BC-producing bacteria have a cellulose synthase operon in their genome. BcsC consists of about 20–30 residues of signal peptides, followed by about 750–900 residues of periplasmic domain of tetratrico peptide repeat (BcsC-TPR), and about 380 residues of the outer membrane domain of the β-barrel (BcsC-C). Thus, the TPR domain is believed to be important for exporting polysaccharides.

In this report, we determined the crystal structure of the N-terminal six TPR motifs in BcsC (BcsC-TPR(N6), Asp24–Arg272) from Enterobacter CJF-002. The crystal structure of BcsC-TPR (Asp24–Arg272) was determined at a resolution of 3.27 Å. There were five molecules in the asymmetric unit and the Matthew’s coefficient was calculated to be 3.9 Å3 Da−1 with a solvent content of 68.5%26. BcsC-TPR(Asp24–Arg272) is a helical structure formed by 14 α-helices (α1–α14). We found a non-TPR α-helix was inserted in the middle of TPR motifs in this structure. A comparison of five monomers in the asymmetric unit showed that they can be classified into three different conformations: chains A and C were type 1 (root mean square deviation (r.m.s.d.) was 0.74 Å for 243 Cα atoms), chains B and D were type 2 (r.m.s.d. was 0.38 Å for 204 Cα atoms), and chain E was type 3. The conformations of these three types were different at the turn region between α5 and α6. The C-terminal two helices (α12–α13) were not included for this calculation since this region was not built for chain E. These results indicate that BcsC-TPR(N6) consists of two structural domains, an N-terminal TPR domain (α1–α5), and a C-terminal TPR domain (α6–α11), connected by a hinge at Thr107–Ala111. Thus, α5 seems to interfere with the formation of the super-helix between TPR2 and TPR3 through the interaction with TPR2. Based on the superposition of types 1 and 3, the C-terminal super-helix changes its screw axis by a conformational change at the loop of Ser109–Gly110. Collectively, the inserted non-TPR region can be considered to play two important roles: covering the interaction region of the upstream TPR motif to separate from the downstream TPR motif, and changing the direction of the downstream super-helix at the loop.

>GHMDEPTAQQQLLSQVRLGEATKREDLVRQSLYRLELIDPDNPDVIAARFRYLLRQGDNAGAQKQLDRMKQLAPDSAAYKSSVTSMTLSGAEGRQALQQARLQATTGHVPEALAAYDALFKGNPPEGDLAVEYWALVAKVPARRSEAITQLKALNARNPGNAALQNSLAQLLFGEGRDAEAYAVLEQMAKSSAGREAAAGLWYQQIQRMPVSDASVKALQRFLTVFSSGDTVDSARTQLAAQQKQLADPAFRLEHHHHHH[5x]> DLLDERGNFSKFTLGDMEMLDVEGVADIDPNYKFNQLLIHNNALSSVLMGSHNGIEPEKVSLLYAGNGGFGDKHDWNATVGYKDQQGNNVATLINVHMKNGSGLVIAGGEKGINNPSFYLYKEDQLTGSQRALSQEEIRNKVDFMEFLAQNNTKLDNLSEKEKEKFQNEIEDFQKDSKAYLDALGNDRIAFVSKKDTKHSALITEFNNGDLSYTLKDYGKKADKALDREKNVTLQGSLKHDGVMFVDYSNFKYTNASKNPNKGVGATNGVSHLEAGFNKVAVFNLPDLNNLAITSFVRRNLENKLTAKGLSLQEANKLIKDFLSSNKELAGKALNFNKAVAEAKSTGNYDEVKKAQKDLEKSLRKREHLEKEVEKKLESKSGNKNKMEAKAQANSQKDEIFALINKEANRDARAIAYTQNLKGIKRELSDKLEKISKDLKDFSKSFDEFKNGKNKDFSKAEETLKALKGSVKDLGINPEWISKVENLNAALNEFKNGKNK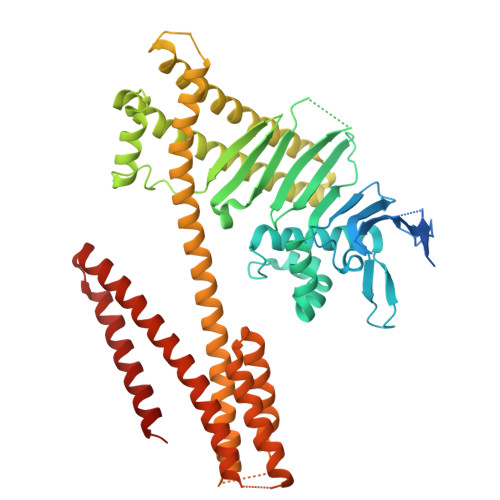DFSKVTQAKSDLENSVKDVIINQKVTDKVDNLNQAVSVAKAMGDFSRVEQVLADLKNFSKEQLAQQAQK>[2x]MKINDDIKELILEYM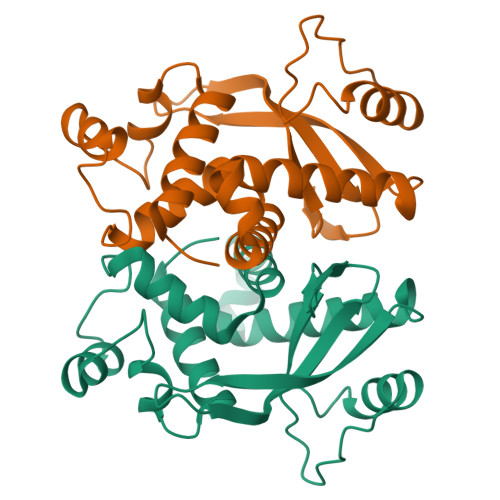SRYFKFENDFYKLPGIKFTDANWQKFKNGGTDIEKMGAARVNAMLDCLFDDFELAMIGKAQTNYYNDNSLKMNMPFYTYYDMFKKQQLLKWLKNNRDDVIGGTGRMYTASGNYIANAYLEVALESSSLGSGSYMLQMRFKDYSKGQEPIPSGRQNRLEWIENNLENIR2-[(2~{R},3~{S},4~{R},5~{R})-5-(hydroxymethyl)-3,4-bis(oxidanyl)-1-[3-[3-(trifluoromethyl)phenyl]propyl]pyrrolidin-2-yl]-~{N}-methyl-ethanamide 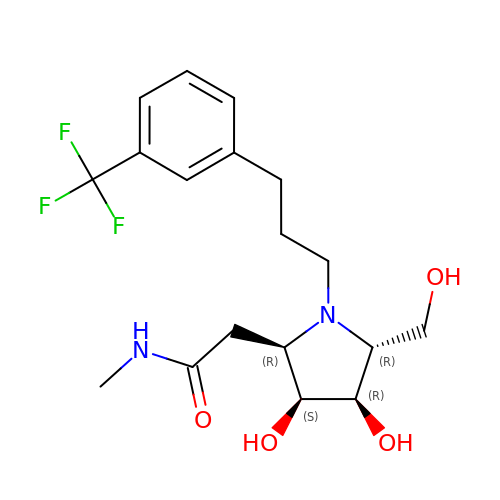| C18 H25 F3 N2 O4 | CCWQIKVWFWMBMG-TXCZRRACSA-N>MIQGVIQKIAGPAVIAKGMLGARMYDICKVGEEGLVGEIIRLDGDTAFVQVYEDTSGLKVGEPVVSTGLPLAVELGPGMLNGIYDGIQRPLERIREKTGIYITRGVVVHALDREKKWAWTPMVKPGDEVRGGMVLGTVPEFGFTHKILVPPDVRGRVKEVKPAGEYTVEEPVVVLEDGTELKMYHTWPVRRARPVQRKLDPNTPFLTGMRILDVLFPVAMGGTAAIPGPFGSGKTVTQQSLAKWSNADVVVYVGCGERGNEMTDVLVEFPELTDPKTGGPLMHRTVLIANTSNMPVAAREASIYVGVTIAEYFRDQGFSVALMADSTSRWAEALREISSRLEEMPAEEGYPPYLAARLAAFYERAGKVITLGGEEGAVTIVGAVSPPGGDMSEPVTQSTLRIVGAFWRLDASLAFRRHFPAINWNGSYSLFTSALDPWYRENVAEDYPELRDAISELLQREAGLQEIVQLVGPDALQDAERLVIEVGRIIREDFLQQNAYHEVDAYCSMKKAYGIMKMILAFYKEAEAAIKRGVSIDEILQLPVLERIGRARYVSEEEFPAYFEEAMKEIQGAFKALA[3x];>[3x]MDLLKKEYTGITYISGPLLFVENAKDLAYGAIVDIKDGTGRVRGGQVIEVSEEYAVIQVFEETTGLDLATTSVSLVEDVARLGVSKEMLGRRFNGIGKPIDGLPPITPEKRLPITGLPLNPVARRKPEQFIQTGISTIDVMNTLVRGQKLPIFSGSGLPANEIAAQIARQATVRPDLSGEGEKEEPFAVVFAAMGITQRELSYFIQEFERTGALSRSVLFLNKADDPTIERILTPRMALTVAEYLAFEHDYHVLVILTDMTNYCEALREIGAAREEIPGRRGYPGYMYTDLATIYERAGVVEGKKGSVTQIPILSMPDDDRTHPIPDLTGYITEGQIQLSRELHRKGIYPPIDPLPSLSRLMNNGVGKGKTREDHKQVSDQLYSAYANGVDIRKLVAIIGEDALTENDRRYLQFADAFERFFINQGQQNRSIEESLQIA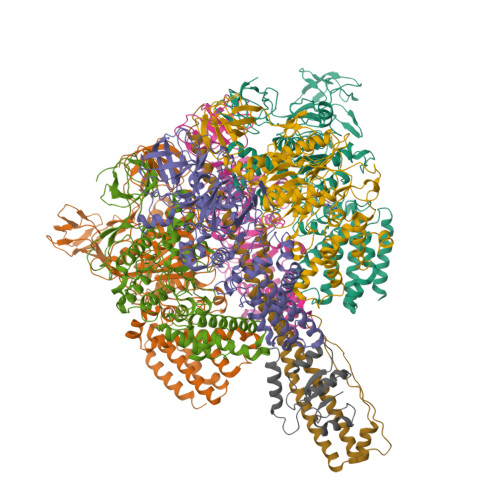WALLSMLPQGELKRISKDHIGKYYGQKLEEIWGAPQALD;> MSQVSPTRMNLLQRRGQLRLAQKGVDLLKKKRDALVAEFFGLVREAMEARKALDQAAKEAYAALLLAQAFDGPEVVAGAALGVPPLEGVEAEVENVWGSKVPRLKATFPDGALLSPVGTPAYTLEASRAFRRYAEALIRVANTETRLKKIGEEIKKTTRRVNALEQVVIPGIRAQIRFIQQVLEQREREDTFRLKRIKGKIEAREAEEEGGRPNPQVEIGAGL;> MAVIADPETAQGFRLAGLEGYGASSAEEAQSLLETLVERGGYALVAVDEALLPDPERAVERLMRGRDLPVLLPIAGLKEAFQGHDVEGYMRELVRKTIGFDIKL>M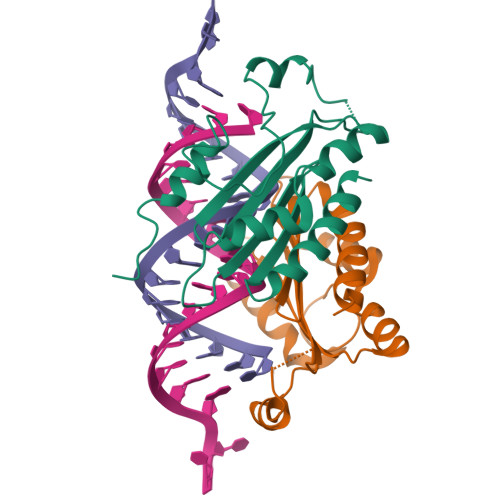ERAIQGNDTREQANGERWDGGSGGITSPFKLPDESPSWTEWRLYNDETNSNQDNPLGFKESWGFGKVVFKRYLRYDRTEASLHRVLGSWTGDSVNYAASRFLGANQVGCSYSIRFRGVSVTISGGSRTLQHLCEMAIRSKQELLQLTPVEVESNVSRGCPEGIETFKKESE[2x]[[(2R,3S,4R,5R)-5-(6-aminopurin-9-yl)-3,4-bis(oxidanyl)oxolan-2-yl]methoxy-oxidanyl-phosphoryl] 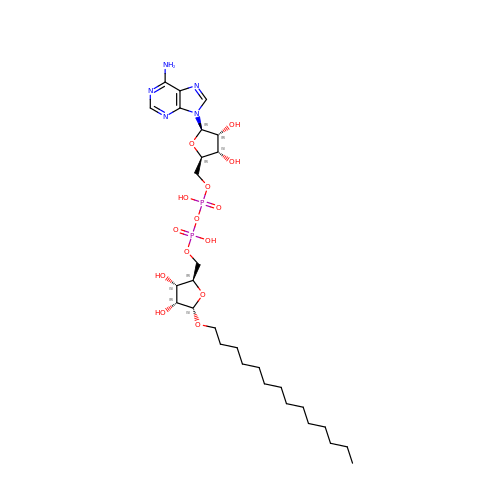[(2R,3S,4R,5S)-3,4-bis(oxidanyl)-5-tetradecoxy-oxolan-2-yl]methyl hydrogen phosphate | C29 H51 N5 O14 P2 | XDVQERDQBQWVRC-UHUMEYFMSA-N>MRGSHHHHHHGSMYLDSQLAERRSMHGVLVDIYGLGVLITGDSGVGKSETALELVQRGHRLIADDRVDVYQQDEQTIVGAAPPILSHLLEIRGLGIIDVMNLFGAGAVREDTTISLIV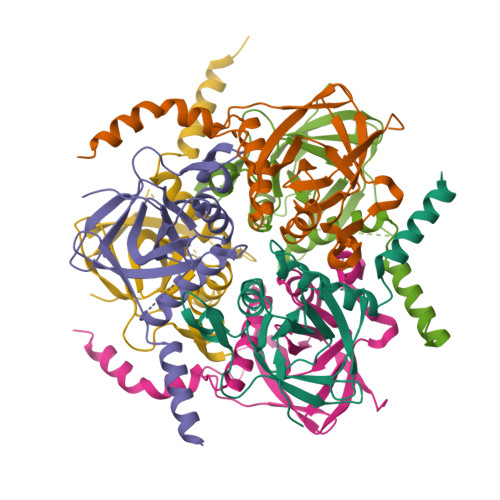HLENWTPDKTFDRLGSGEQTQLIFDVPVPKITVPFKVGRNLAIIIEVAAMNFRAKSMGYDATKTFEKNLNHLIEHNEETDQNSSGDK[12x]>MVRTTKTSMAAASTVAPEVAMDEGSPSTSQAQVELPRNLEVFNEACGHVFGSSFNREDNSVISDAAAFLFKMHTHSLDGQEAKVLRASEKKRERENAKKSRKAPEAGMRVGRSLILTSRWTEYCATCVPALGSKMKVIKASGDAAMIQMMKDHNSLLRVCVRIEVWKARYVSLVALDERIQTLEDAQWFPYLSGDSYRACPGLVGGYFAKKAAAGERGKNYKKLNQTAIIPPPRFLIIGHRLQIGDQVTLRELLASIAWGLCDG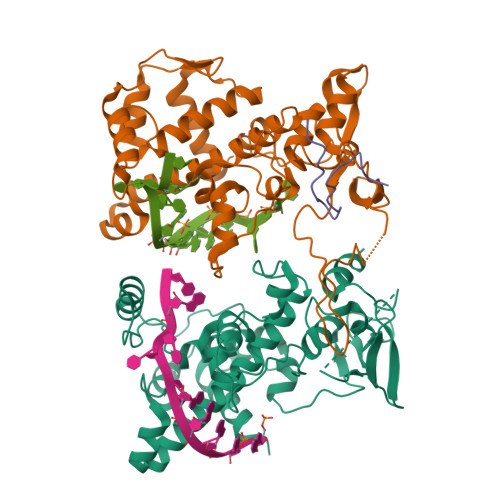VLAECWSPSQGDGSIGVVVGLPLQATGSCFLVVASHGLSAIADSRIEGTGNTNLLEECIAIQKQDGVIKCKRSGKSLYHCLKETAGAVGR[3x]MLKL is a key player in the necroptosis pathway, encompassing a C-terminal regulatory and an N-terminal executioner domain. It gets activated through phosphorylation of Thr357 and Ser358 in its pseudokinase domain by RIP3 kinase and subsequently oligomerizes via its executioner domain and inserts into the membrane. To this end, displacement of the auto-inhibitory brace helix (α-helix 6) from the four-helix bundle is required, which depends on a specific composition of phospholipids in the membrane. Currently, two classes of compounds are reported to inhibit MLKL by covalently binding to Cys86 in the short α-helix 4 located on top of the four-helix bundle, which comprises α-helices 1, 2, 3, and 5.

First, we solved the structure of the unliganded MLKL executioner domain by X-ray crystallography and NMR spectroscopy to have a basis for detailed analysis of structural changes induced by small-molecule binding. Both structures of the unliganded four-helix bundle were highly similar (rmsd value 2.1 Å) and showed only minor differences from the two published NMR solution structures [NMR structure has an rmsd of 2.4 Å to 2MSV and an rmsd of 2.5 Å to 6D74 (12)]. The four-helix bundle was formed by α-helices 1, 2, 3, and 5 of MLKL with a short interjacent α-helix 4 on top. The flexible linker between α-helices 5 and 6 (residues 120 to 130) was not fully visible in the X-ray structures due to inherent flexibility. The subsequent α-helix 6 packed with multiple contacts, against the four-helix bundle. The 1H,15N-correlation spectrum of the unliganded MLKL four-helix bundle showed only one peak for the Hε1–Nε1 correlation of Trp133, consistent with its side chain packed between α-helices 2 and 5 and, thereby, anchoring α-helix 6 to the four-helix bundle. The unliganded MLKL executioner domain had a hydrodynamic radius of 19 Å, which is consistent with a monomer.

>[3x]GSPGENLKHIITLGQVIHKRCEEMKYCKKQCRRLGHRVLGLIKPLEMLQDQGKRSVPSEKLTTAMNRFKAALEEANGEIEKFSNRSNICRFLTASQDKILFKDVNRKLSDVWKELSLLLQVEQRMPVSPISQGASWAQEDQQDADEDRRAFQM> GSGAPPTIQQPSMSSAVALLGQDVDFTCIVNDLGSHMVAFVKADSPPRLLSFDEKVFRRRNKYELKPRIGDLHNEWVLTIKNVQESDRGNYSCQINTEPITLS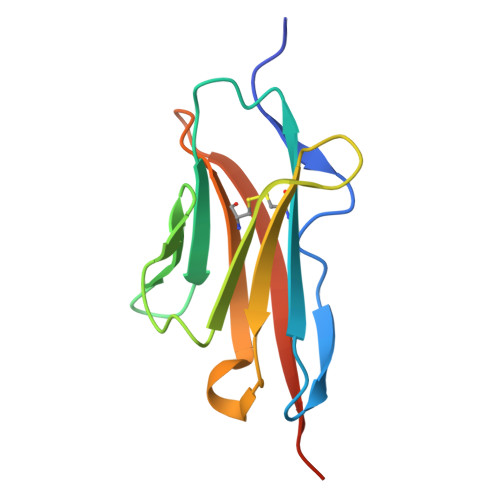TGELDVKVPHHHHHH> QQVGTQTAENHPKLTVSQCSAGGSCTTESRSVVLDSNW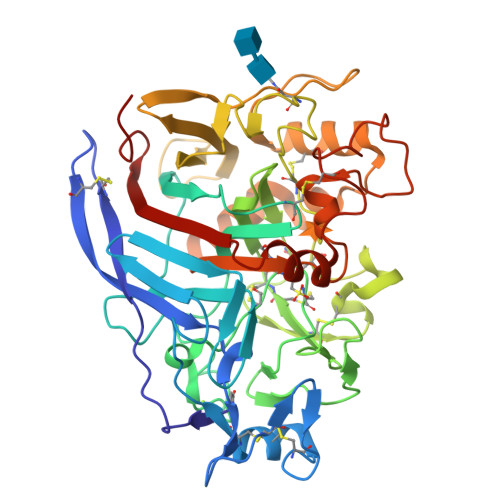RWLHTTSGTTNCYTGNTWDASLCPDPVTCAQNCALDGADYSGTYGISTSGNALTLKFVTNGPYSTNIGSRVYLMSADDTNYEIFKLKNQEFAFDVDMSNLPCGLNGALYFVEMDADGGLSRFPNNKAGSKYGTGYCDTQCPQDIKFINGEANILGWTPSSSDSNAGTGQYGSCCNEMDVWEANINSAAVTPHVCNVQGQTRCSGTQCGDGDERYDGICDKDGCDFNSFRMGNQTFLGPGKTVNTNSKFTVVTQFLTSDNTTTGTLHEIRRLYVQNGKVIANSKTNIAGMSQFDSITDDFCNAQKTAFGDTNSFENLGGLNVMGQAFDKGVVLVMSVWDDHEANMLWLDSDYPTTSSASTPGVARGTCATTSGVPANVESQNPNSSVVFSNIKIGPIGSTYTA> REATWVTEKPLTLKIHMHFRDKWVWDENWPVAREVARLTNVKLVGVANRAATNSQEQFNLMMASGQLPDIVGGDNLKDKFIRYGMEGAFIPLNKLIDQNAPNLKAFFKTHPEVQRAITAPDGNIYYLPYVPDGLVSRGYFIRQDWLDKLHLKTPQTVDELYTVLKAFKEKDPNGNGKADEIPFINRDPEEVFRLVNFWGARSTGSNTWMDFYVENGKIKHPFAEVAFKDGIKHVAQWYKEGLIDPEIFTRKARSREQTFGNNIGGMTHDWFASTALFNDALSKNIPGFKLVPMAPPINSKGQRWEEDARQIPRPDGWAITATNKNPVETIKLFDFYFGPKGRELSNFGVPGLTYDIKNGKPVYKDTVLKAAQPVNNQMYDIGAQIPIGFWQDYEYERQWTNDVALQGIDMYIKNKYVLPQFTGVNLTVEEREIYDKYWPDVKTYMFEMGQSWVMGTKDPEKTWNDYQQQLKNRGFYQVMIVMQKAYD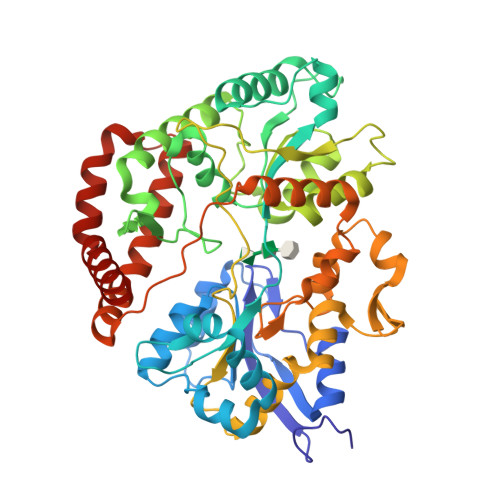RQY> GSHMDKLPIEETLEDSPQTRSLLGVFEEDATAISNYMNQLYQAMHRIYDAQNELSAATHLTSKLL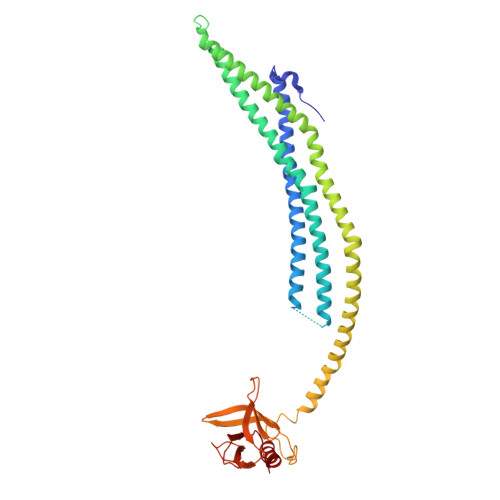KEYEKQRFPLGGDDEVMSSTLQQFSKVIDELSSCHAVLSTQLADAMMFPITQFKERDLKEILTLKEVFQIASNDHDAAINRYSRLSKKRENDKVKYEVTEDVYTSRKKQHQTMMHYFCALNTLQYKKKIALLEPLLGYMQAQISFFKMGSENLNEQLEEFLANIGTSVQNVRREMDSDIETMQQTIEDLEVASDPLYVPDPDPTKFPVNRNLTRKAGYLNARNKTGLVSSTWDRQFYFTQGGNLMSQARGDVAGGLAMDIDNCSVMAVDCEDRRYCFQITSFDGKKSSILQAESKKDHEEWICTINNISK Forkhead box H1 (FoxH1) is an essential maternal pioneer factor during embryonic development that binds to specific GG/GT-containing DNA target sequences. The members of the FOX transcription factor family share the presence of the forkhead domain (FH), which interacts with DNA (InterPro entry IPR001766). Most FOX proteins recognize the canonical forkhead DNA motif TRTTTRY (R = A/G, Y = C/T). In contrast, FoxH1 recognizes the TGTG(G/T)ATT sequences in several cis-regulatory elements, such as in Gsc, Eomes, Nodal, Mixl, and FoxA2, to confer activin regulation in vivo.

In contrast, FoxA2, also a pioneer factor that binds to canonical forkhead motifs, displayed the opposite behavior and selected only for DNAs with TT sites, even showing a decrease in its melting temperature in the presence of the GG site. Also, EMSA assays indicated that FoxA2 binds weakly to the TGTGGATT site whereas it interacts with high affinity with its forkhead site. We observed that only high FL-FoxH1 concentrations could displace FoxA2 from the DNA. These findings corroborate that FoxH1 and FoxA2 interact with TT sites, although the former has the distinct ability to recognize GK sites, a rare feature among FOX proteins. To explore the impact of the protein-DNA interactions on the DNA topology, we compared the DNA shapes of the FoxH1 complexes with other FOX structures available in the PDB and with the pair of complexes we determined here for FoxA2 using Curves+ 43. Small differences were detected at the major groove, whereas the minor grooves were found to be slightly wider in the FoxH1 complexes than in other FOX structures. A similar absence of interaction between Asn and the G-C pair could account for the DNA binding preferences of FoxA2. The structural information we gathered for the DNA binding specificities of FoxA2 and FoxH1 FH domains is compatible with the hypothesis whereby FoxA proteins substitutes for FoxH1 preferentially at TT sites, with FoxH1 remaining bound to GK sites even when the concentration of this protein is low.

> KTYRRSYTHAKPPYSYISLITMAIQQSPNKMLTLSEIYQWIMDLFPFYRQNQQRWQNSIRHSLSFNDCFLKVPRSPDKPGKGSFWTLHPDSGNMFENGCYLRRQKRFKCEKQLALKEAAGAAGSG> MFKAQATFSRYSAAVSLLLLFSGAAQAAPQSITTLPLQPDGENRWRLPAGEYQGQFTIEQPMQLRCEPGAVIQSQGQGSSLLISAPDVLVEGCTLYEWGSDLTAMDSAVFILPAAERAQISNNRMRGPGFGVFVDGTRDVQVIGNEIDGDAGVRSQDRGNGIHLFAVSGARVLHNHVRNARDGIYIDTSNGNHLEGNVIEDVRYGVHYMFANENSLIDNVTRRTRTGYALMQSRKLTVTGN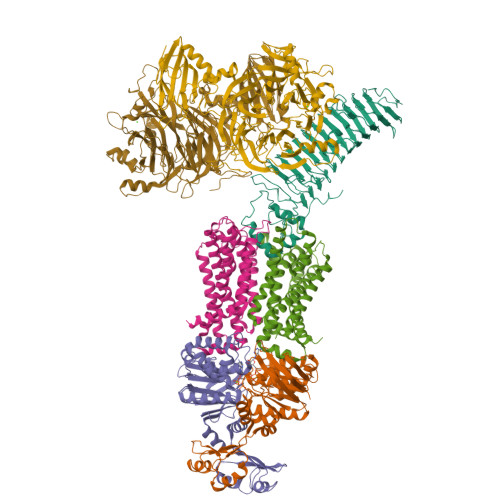RSEQDQNYGILMNYITYSTITGNFVSDVQRGDTGGDSMISGGEGKALFIYNSLFNTIENNHFEKSSLGIHLTAGSEDNRISGNAFVGNQQQVKYVASRTQEWSVDGRGNYWSDYLGWDRNNDGLGDIAYEPNDNVDRLLWLYPQVRLLMNSPSIEVLRWVQRAFPVIKSPGVQDSHPLMKLPTEKLLTEKQEPTS;>[2x]HHHHHHNAVEIQGVSQRYGSMTVLHDLNLNLGEGEVLGLFGHNGAGKTTSMKLILGLLSPSEGQVKVLGRAPNDPQVRRQLGYLPENVTFYPQLSGRETLRHFARLKGAALTQVDELLEQVGLAHAADRRVKTYSKGMRQRLGLAQALLGEPRLLLLDQPTVGLDPIATQDLYLLIDRLRQRGTSIILCSHVLPGVEAHINRAAILAKGCLQAVGSLSQLRAEAGLPVRIRASGISERDSWLQRWTDAGHSARGLSESSIEVVAVNGHKLVLLRQLLGEGEPEDIEIHQPSLEDLYRYYMERAGDVRAQEGRL;>[2x]MNQVWNIARKELSDGLRNRWLLAISLLFAVLAVGIAWLGAAASGQLGFTSIPATIASLASLATFLMPLIALLLAYDAIVGEDEGGTLMLLLTYPLGRGQILLGKFVGHGLILALAVLIGFGCAALAIALLVEGVELGMLFWAFGRFMISSTLLGWVFLAFAYVLSGKVNEKSSAAGLALGVWFLFVLVFDLVLLALLVLSEGKFNPELLPWLLLLNPTDIYRLINLSGFEGSGSAMGVLSLGADLPVPAAVLWLCLLAWIGVSLLLAYAIFRRRLT;>[2x]MSDKDSKNTPQVPEKLGLSRRGFLGASAVTGAAVAATALGGAVMTRESWAQAVKESKQKIHVGPGELDDYYGFWSGGHQGEVRVLGVPSMRELMRIPVFNVDSATGWGLTNESRHIMGDSAKFLNGDCHHPHISMTDGKYDGKYLFINDKANSRVARIRLDIMKCDKMITVPNVQAIHGLRLQKVPHTKYVFANAEFIIPHPNDGKVFDLQDENSYTMYNAIDAETMEMAFQVIVDGNLDNTDADYTGRFAAATCYNSEKAFDLGGMMRNERDWVVVFDIHAVEAAVKAGDFITLGDSKTPVLDGRKKDGKDSKFTRYVPVPKNPHGCNTSSDGKYFIAAGKLSPTCSMIAIDKLPDLFAGKLADPRDVIVGEPELGLGPLHTTFDGRGNAYTTLFIDSQVVKWNMEEAVRAYKGEKVNYIKQKLDVHYQPGHLHASLCETNEADGKWLVALSKFSKDRFLPVGPLHPENDQLIDISGDEMKLVHDGPTFAEPHDCIMARRDQIKTKKIWDRNDPFFAPTVEMAKKDGINLDTDNKVIRDGNKVRVYMTSMAPAFGVQEFTVKQGDEVTVTITNIDQIEDVSHGFVVVNHGVSMEISPQQTSSITFVADKPGLHWYYCSWFCHALHMEMVGRMMVEPAWSHPQFEK>[2x]DPAGADAGSAVPFHGAHQAGIATPVQDRLHFAAFDVTTEDRAAFVALLKEWTAAARR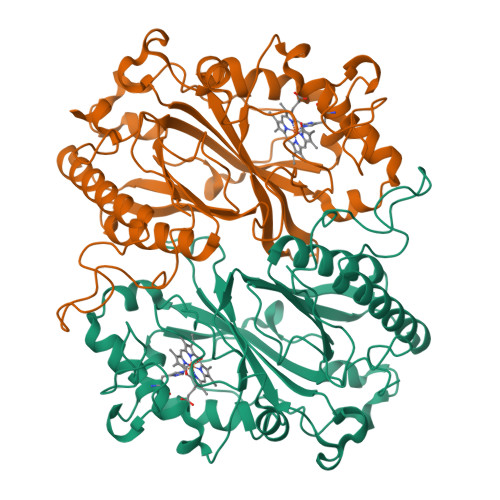LTAGHAVGEGAYGGLPEAPPDDTGEALGLKPSRLTLTIGFGPSLFTRFGLADLRPEALADLPKFPGDNLDRARSGGDLCVQACADDPQVAVHAIRNLARIGFGKVVVRWSQLGFGKTSSTTPDKQTPRNLLGFKDGTRNIAGTEKDRLDRFVWAAEKDGTPWMTGGSYLVARRIRMHIETWDRASLQEQEDVFGRDKGEGAPVGKAKERDEPFLKAMKPDAHVRLAHPDSNGGATLLRRGYSFTDGTDGLGRLDAGLFFLAYQRDIRTGFVPVQRNLATDALNEYIQHVGSAVFAVPPGVRDADDWWGSTLFGKEA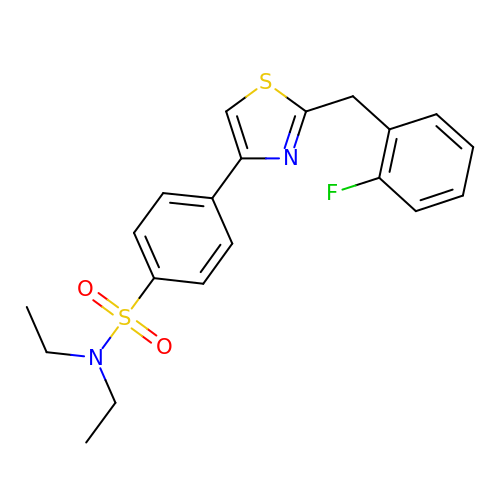N,N-diethyl-4-{2-[(2-fluorophenyl)methyl]-1,3-thiazol-4-yl}benzene-1-sulfonamide | C20 H21 F N2 O2 S2 | PZNJPNGENGJLBG-UHFFFAOYSA-N6-({5-[(3aS,4S,5S,6aR)-5-oxido-2-oxohexahydro-1H-thieno[3,4-d]imidazol-4-yl]pentanoyl}amino)hexanoic 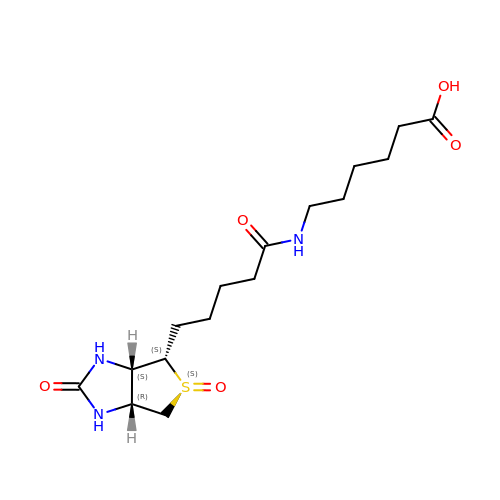acid | C16 H27 N3 O5 S | WVGTVVXHODUEJR-XNCOPMLMSA-N>[2x]MVLYFIGLGLYDERDITVKGLEIAKKCDYVFAEFYTSLMAGTTLGRIQKLIGKEIRVLSREDVELNFENIVLPLAKENDVAFLTPGDPLVATTHAELRIRAKRAGVESYVIHAPSIYSAVGITGLHIYKFGKSATVAYPEGNWFPRSYYDVIKENAERGLHTLLFLD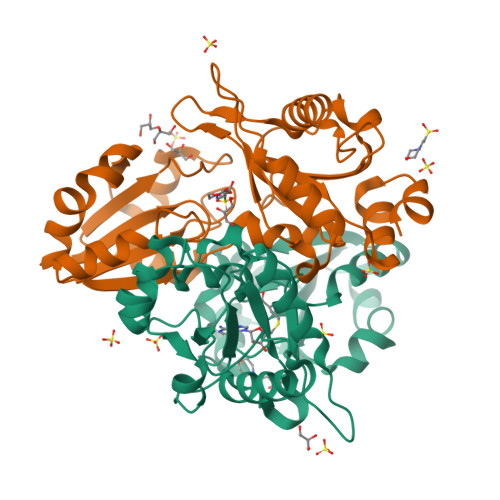IKAEKRMYMTANEAMELLLKVEDMKKGGVFTDDTLVVVLARAGSLNPTIRAGYVKDLIREDFGDPPHILIVPGKLHIVEAEYLVEIAGAPREILRVNV>MGFKEYPAGEPVTMNEMELAAVYLQPIDMEPRGMGLPAAKADVHLEADIHAVEGNKNGFGAGEWIPYLTISYTLVNNDTGEKQEGTFMPMVASDGPHYGANIKMMGVGNYKVTYHIE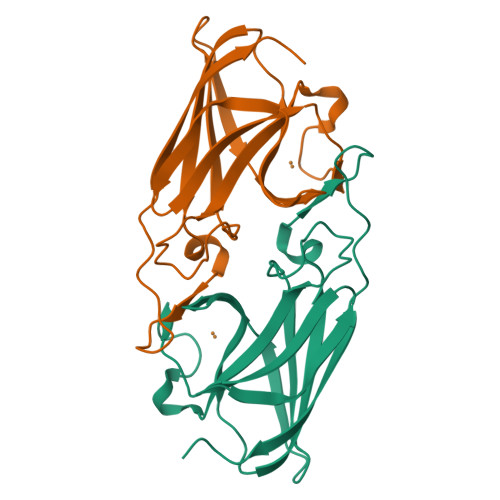PPSKAGMHRHTDSETGVGRWWKPFDVSYEFKYVGLNSSGLVPR[2x]>[4x]MRGSHHHHHHGSMPVAGSELPRRPLPPAAQERDAEPRPPHGELQYLGQIQHILRCGVRKDDRTGTGTLSVFGMQARYSLRDEFPLLTTKRVFWKGVLEELLWFIKGSTNAKELSSKGVKIWDANGSRDFLDSLGFSTREEGDLGPVYGFQWRHFGAEYRDMESDYSGQGVDQLQRVIDTIKTNPDDCRIIMCAWNPRDLPLMALPPCHALCQFYVVNSELSC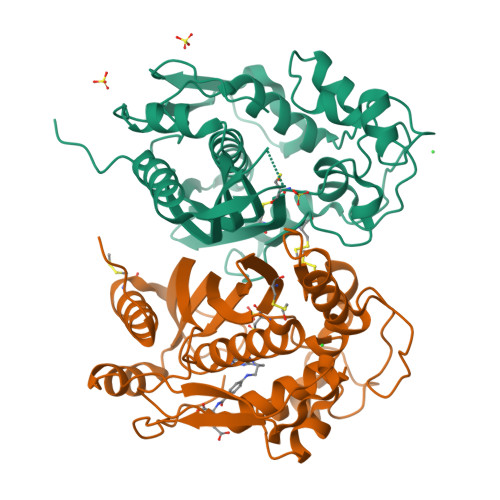QLYQRSGDMGLGVPFNIASYALLTYMIAHITGLKPGDFIHTLGDAHIYLNHIEPLKIQLQREPRPFPKLRILRKVEKIDDFKAEDFQIEGYNPHPTIKMEMAV>TVVEEPVDITPYLDQLDESLRDKVLQLQKGSDTEAQCEVMQEIVDQVLEEDFD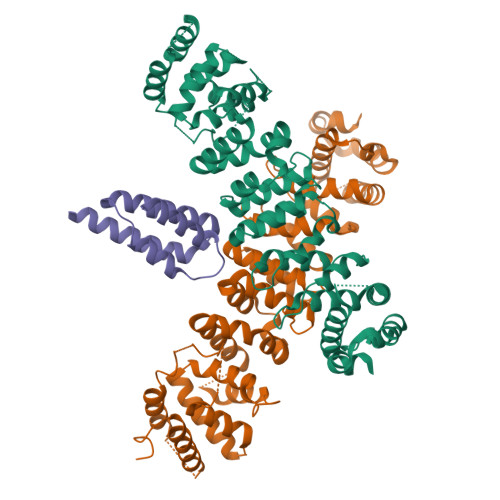SEQLSVLASCLQELFKAHFRGEVLPEEITEESLEESVGKPLYLIFRNLCQMQEDNSSFSLLLDLLSELYQKQPKIGYHLLYYLRASKAAAGKMNLYESFAQATQLGDLHTCLMMDMKACQEDDVRLLCHLTPSIYTEFPDETLRSGELLNMIVAVIDSAQLQELVCHVMMGNLVMFRKDSVLNILIQSLDWETFEQYCAWQLFLAHNIPLETIIPILQHLKYKEHPEALSCLLLQLRREKPSEEMVKMVLSRPCHPDDQFTTSILRHWCMKHDELLAEHIKSLLIKNNSLPRKRQSLRSSSSKLAQLTLEQILEHLDNLRLNLTNTKQNFFSQTPILQALQHVQASCDEAHKMKFSDLFSLAEEYEDSSTKPPKSRRKAALSS[2x];> MHCRSHEEVNTELKAQIMKEIRKPGRKYERIFTLLKHVQGSLQTRLIFLQNVIKEASRFKKRMLIEQLENFLDEIHRRANQINHINSN> MTQQPLRGVTSLRFNQDQSCFCCAMETGVRIYNVEPLMEKGHLDHEQVGSMG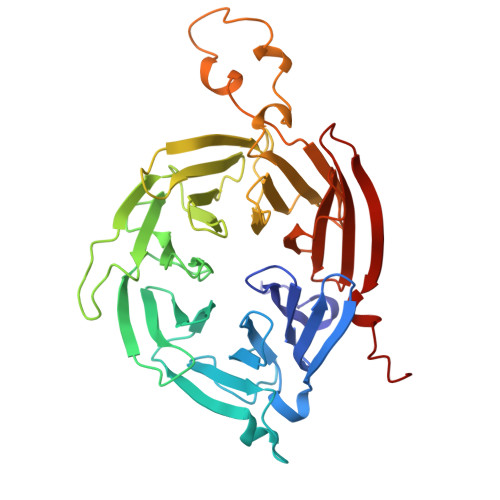LVEMLHRSNLLALVGGGSSPKFSEISVLIWDDAREGKDSKEKLVLEFTFTKPVLSVRMRHDKIVIVLKNRIYVYSFPDNPRKLFEFDTRDNPKGLCDLCPSLEKQLLVFPGHKCGSLQLVDLASTKPGTSSAPFTINAHQSDIACVSLNQPGTVVASASQKGTLIRLFDTQSKEKLVELRRGTDPATLYCINFSHDSSFLCASSDKGTVHIFALKDTRLNRRSALARVGKVGPMIGQYVDSQWSLASFTVPAESACICAFGRNTSKNVNSVIAICVDGTFHKYVFTPDGNCNREAFDVYLDICDDDDF> LRQCLPCGPGGKGRCFGPSICCGDELGCFVGTAEALRCQEENYLPSPCQSGQKPCGSGGRCAA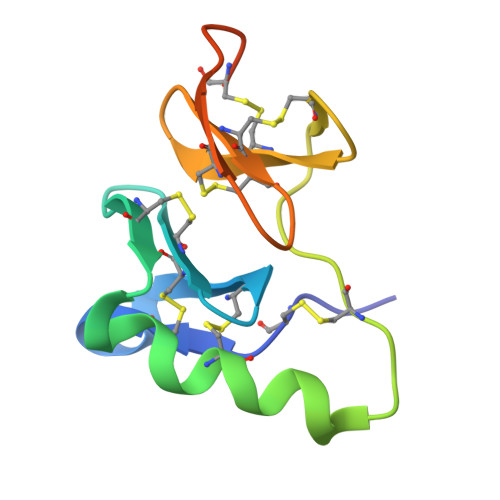AGICCNDESCVTEPECREGVGFPRRV alpha-D-galactopyranuronic 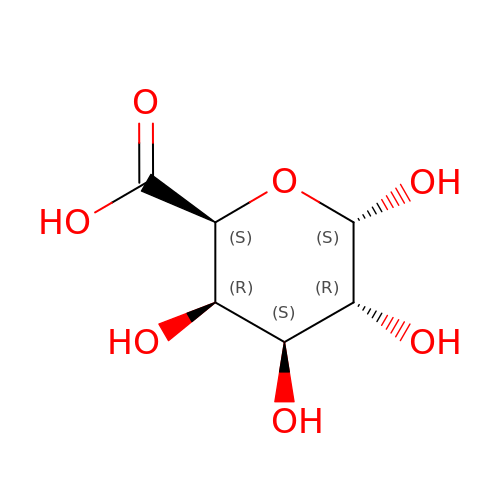acid | C6 H10 O7 | AEMOLEFTQBMNLQ-BKBMJHBISA-N> MTIKEDGMSETQYFVSHDGNRHDLFDTLEQAEHYILKKNGWTDGEIAEKWAFVKKEARKYGGDPFSSNGRHSLWFITELKLSDGVIMEVDGQLFDDYVESISAERGTEEFAE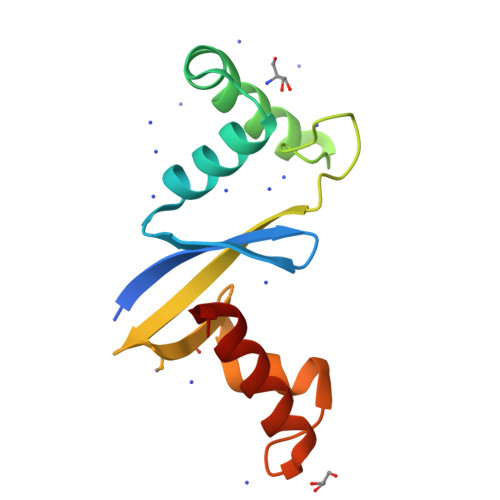TKRRLVGYYLGW>[12x]MFERFTDRARRVVVLAQEEARMLNHNYIGTEHILLGLIHEGEGVAAKSLESLGISLEGVRSQVEEIIGQGQQAPSGHIPFTPRAKKVLELSLREALQLGHNYIGTE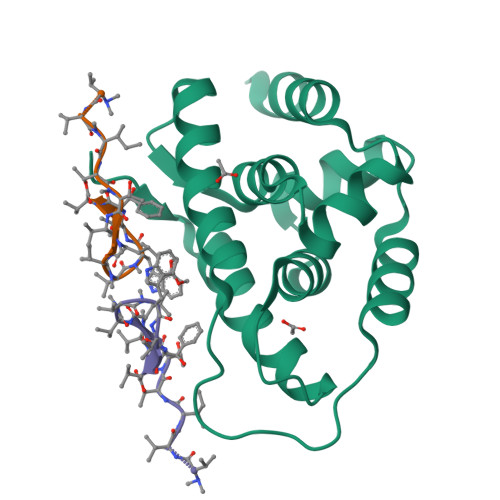HILLGLIREGEGVAAQVLVKLGAELTRVRQQVIQLLSGYKLAAALEHHHHHH>MNLTELKNTPVSELITLGENMGLENLARMRKQDIIFAILKQHAKSGEDIFGDGVLEILQDGFGFLRSADSSYLAGPDDIYVSPSQIRRFNLRTGDTISGKIRPPKEGERYFALLKVNEVNFDKPENARNKILFENLTPLHANSRLRMERGNGSTEDLTARVLDLASPIGRGQRGLIVAPPKAGKTMLLQNIAQSIAYNHPDCVLMVLLIDERPEEVTEMQRLVKGEVVASTFDEPASRHVQVAEMVIEKAKRLVEHKKDVIILLDSITRLARAYNTVVPASGKVLTGGVDANALHRPKRFFGAARNVEEGGSLTIIATALIDTGSKMDEVIYEEFKGTGNMELHLSRKIAEKRVFPAIDYNRSGTRKEELLTTQEELQKMWILRKIIHPMGEIDAMEFLINKLAMTKTNDDFFEMMKRS[6x];>AMGNDTYQPINCDDYDNLELACQHHLMLTLELKDGEKLQAKASDLVSRKNVEYLVVEAAGETRELRLDKITSFSHPEIGTVVVSES[5x]

Bacterial transcription termination factor, ρ, is a hexameric, NTP-dependent 5’–3’ RNA translocase and helicase. A ρ monomer contains N-terminal (NTD) and C-terminal (CTD) domains connected by a flexible linker. The NTD comprises an N-terminal three-helix bundle and a five-stranded β-barrel, the OB-fold, that forms a primary RNA-binding site (PBS); the PBSes are located around one outer rim of the ρ hexamer. The CTDs jointly form a secondary RNA-binding site (SBS) at the center of the ρ hexamer.

We subjected SEC fractions corresponding to ρ-Rof complexes to cryoEM/SPA in the absence and presence of the transition state analog, ADP-BeF3. In the first assembly, ρ forms an open hexameric ring (ρA-ρF) bound by five Rof molecules (Rofa-Rofe), while the second assembly represents a ρ pentamer (ρA-ρE) bound by four Rof molecules (Rofa-Rofd). In the presence of ADP-BeF3, we obtained a ~1:1 (ρ6-Rof5:ρ5-Rof4) distribution between the two classes, whereas in the absence of the nucleotide, the equilibrium was shifted towards the lower oligomeric assembly (ρ6-Rof5:ρ5-Rof4 ~ 1:3). We built an initial atomic model of ρ-bound Rof based on the density for Rofc in the ρ6-ADP-Rof5 structure, which is best defined. We therefore focus our subsequent descriptions on the ρ6-ADP-Rof5 complex and on Rofc when discussing interaction details. In each case, Rof interacts primarily with one ρ NTD through its N-terminal α-helix (α1, residues 9–23), the loop connecting strands β3 and β4 (residues 46–50) and the very C-terminal region. In addition, loopβ3-β4 of Rof contacts the N-terminal three-helix bundle of the adjacent ρ protomer, presumably explaining why Rof binding is only observed between neighboring ρ subunits but not at the terminal subunits of the open ring. The N-terminus and helix α1 of Rof are positioned in a cavity of the ρ NTD between ρ helix α4 (residues 83–89) and one flank of the ρ OB-fold (residues 95–120). Surprisingly, although ρ adopts an open conformation upon Rof binding, the connector retains the NTD/CTD-interaction register of the closed conformation, presumably due to the direct Rof-helix α5 interactions restricting connector rearrangements. Concomitantly, in complex with Rof, the CTD Q-loops adopt a conformation observed in closed ρ, but not in open ρ structures in the absence of Rof 42; in the closed ring as well as in the open ring in complex with Rof, ρK283 is inserted into a pocket formed by the Q-loop of the adjacent protomer, while ρK283 points to the center of the ring in open ρ in the absence of Rof.>[2x]AAESGARSVCNTVRRRSAGMLRKDSQDASDEKYVRGCYFTNWAQYRPGNGKYNPEHYQANLCEYIFYAFAKLNDDFTVDQFEWNDIDVLYPGVMKQKSSQPDLKVLLSLGGWNAGTATFKKMAATYSNRAKFISSLVSFLQQNKFDGF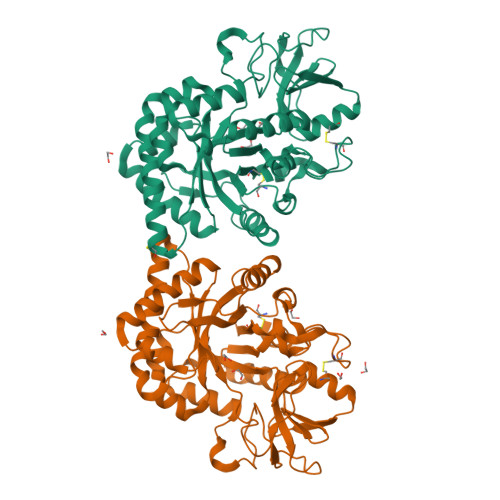DLDWEYPESSDKENYLLLCQEILAKFEEVAKCTSTSRLLFTAAVSANPKTVDAGYDVPALAKVLDFVNLMCYDFHGAWETQTGINSPLYSRKEDSSEFKMWNVEQSSKYWSDKGMPKKQIIIGLPTYGRGWTLSDASKTDIGAPAQGSSTATEYLREAGVISYYEVCQKLSSGAKRVWDDESKTPYLVQGNQWFSYDDVESMKAKINWIKQENYGGAFVWTLDYDDFLGSFCTEHNGKKYPLISLMQEILGGGYVPPSTESTTSQVTTTPSTTTSTTSPAGAFQCPSDGLFPDPESCSNFYQCAGGTAYKMKCPTGLMFNPKTSTCDYPSNVDCQEKTITTHHHHHH>[4x]GGVDREAMARCIEECLRCAQ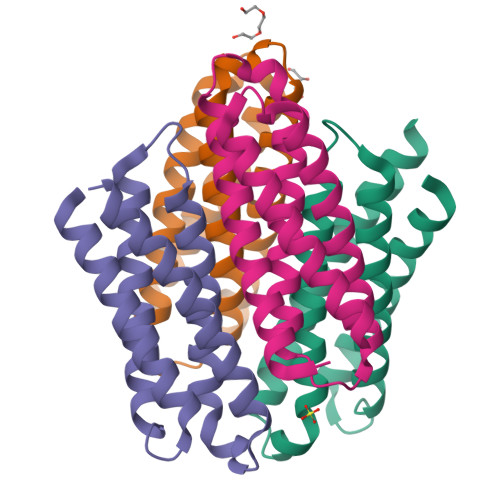ACTACADACLSEPTVADLTKCIRTDMDCADVCTATAAVLSRHTGYDANVTRAVLQACATVCAACGDECARHAGMHEHCRVCAEACRSCEQACQELLAGL> GPLGSMSFLKTVPEELTAAAAQLGTIGAAMAAQNAAAAAPTTAIAPAALDEVSALQAALFTAYGTFYQQVSAEAQAMHDMFVNTLGISAGT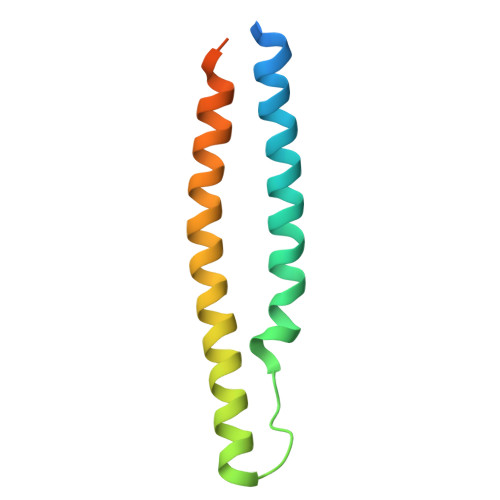YGVTESLNSSAAA>HHHHHHASMDKNIIIGAMTALITPFKNGKVDEQSYARLIKRQIENGIDAVVPVGTTGESATLTHEEHRTCIEIAVETCKGTKVKVLAGAGSNATHEAVGLAKFAKEHGADGILSVAPYYNKPTQQGLYEHYKAIAQSVDIPVLLYNVPGRTGCEISTDTIIKLFRDCENIYGVKEASGNIDKCVDLLAHEPRMMLISGEDAINYPILSNGGKGVISVTSNLLPDMISALTHFALDENYKEAKKINDELYNINKILFCESNPIPIKTAMYLAGLIESL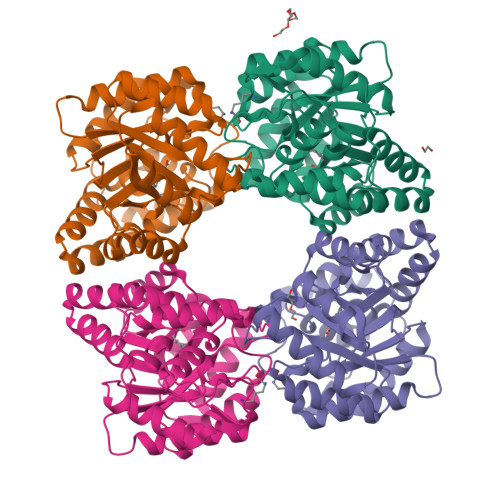EFRLPLCSPSKENFAKIEEVMKKYKIKGF[4x]>[4x]MSE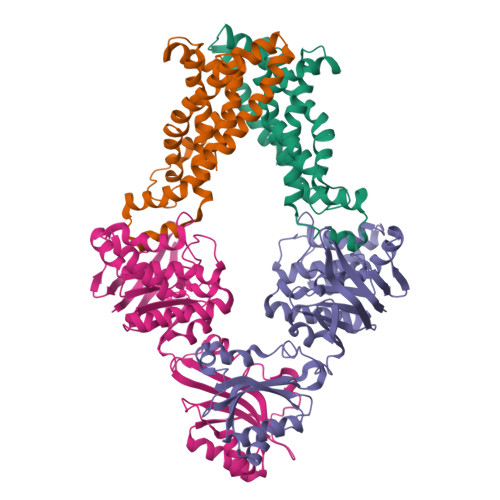PMMWLLVRGVWETLAMTFVSGFFGFVIGLPVGVLLYVTRPGQIIANAKLYRTVSAIVNIFRSIPFIILLVWMIPFTRVIVGTSIGLQAAIVPLTVGAAPFIARMVENALLEIPTGLIEASRAMGATPMQIVRKVLLPEALPGLVNAATITLITLVGYSAMGGAVGAGGLGQIGYQYGYIGYNATVMNTVLVLLVILVYLIQFAGDRIVRAVTRK;>MIKLSNITKVFHQGTRTIQALNNVSLHVPAGQIYGVIGASGAGKSTLIRCVNLLERPTEGSVLVDGQELTTLSESELTKARRQIGMIFQHFNLLSSRTVFGNVALPLELDNTPKDEVKRRVTELLSLVGLGDKHDSYPSNLSGGQKQRVAIARALASNPKVLLCDEATSALDPATTRSILELLKDINRRLGLTILLITHEMDVVKRICDCVAVISNGELIEQDTVSEVFSHPKTPLAQKFIQSTLHLDIPEDYQERLQAEPFTDCVPMLRLEFTGQSVDAPLLSETARRFNVNNNIISAQMDYAGGVKFGIMLTEMHGTQQDTQAAIAWLQEHHVKVEVLGYV[4x]>[2x]GVIKPDMKIKLKMEGNVNGHAFVIEGEGEGKPYDGTNTINLEVKEGAPLPFSYD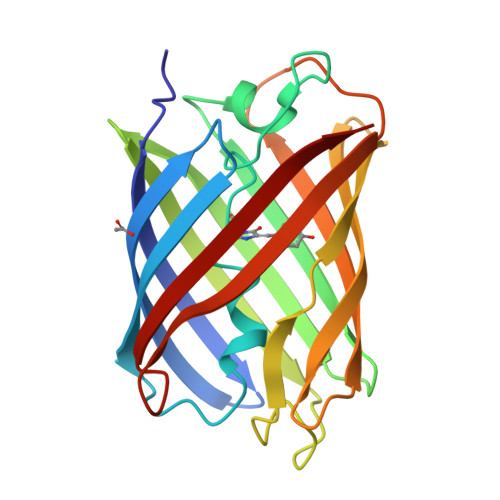ILTNAFAYGNRAFTKYPDDIPNYFKQSFPEGYSWERTMTFEDKGIVKVKSDISMEEDSFIYEIHLKGENFPPNGPVMQKKTLKWEPSTEILYVRDGVLVGDIKHKLLLEGGGHHRVDFKTIYRAKKAVKLPDYHFVDHRIEILNHDKDYNKVTVYESAVARY>[3x]MVNNNRPRRQRAQRVVVTTTQTAPVPQQNVPRNGRRRRNRTRRNRRRVRGMNMAALTRLSQPGLAFLKCAFAPPDFNTDPGKGIPDRFEGKVVSRKDVLNQSISFTAGQDTFILIAPTPGVAYWSASVPAGTFPTSATTFNPVNYPGFTSMFGTTSTSRSDQVSSFRYASMNVGIYPTS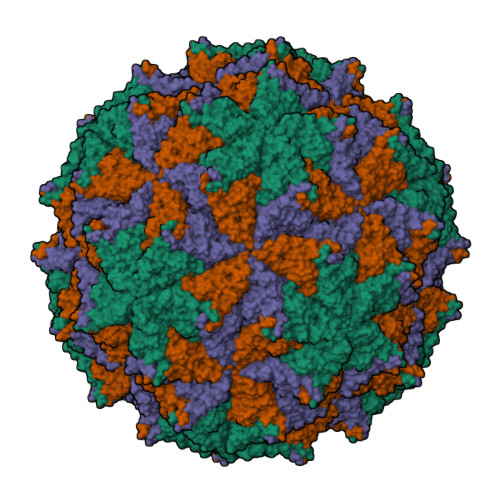NLMQFAGSITVWKCPVKLSTVQFPVATDPATSSLVHTLVGLDGVLAVGPDNFSESFIKGVFSQSACNEPDFEFNDILEGIQTLPPANVSLGSTGQPFTMDSGAEATSGVVGWGNMDTIVIRVSAPEGAVNSAILKAWSCIEYRPNPNAMLYQFGHDSPPLDEVALQEYRTVARSLPVAVIAAQN;>ASMWERVKSIIKSSLAAASNIPGPIGVAASGISGLSALFEGFGF[3x]> MATANNPPSGLLDPTLCEDRIFYNILEIEPRFLTSDSVFGTFQQSLTSHMRKLLGTWMFSVCQEYNLEPNVVALALNLLDRLLLIKQVSKEHFQKTGSACLLVASKLRSLTPISTSSLCYAAADSFSRQELIDQEKELLEKLAWRTEAVLATDVTSFLLLKLVGGSQHLDFWHHEVNTLITKALVDPLTGSLPASI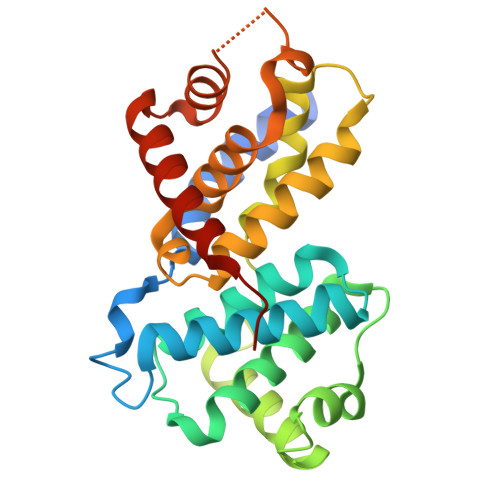ISAAGCALLVPANVIPQDTHSGGVVPQLASILGCDVSVLQAAVEQILTSVSDFDLRILDSY>QLNPYLRLKVRRDHIIDDALVRLEMIAMENPADLKKQLYVEFEGEQGVDEGGVSKEFFQLVVEEIFNPDIGMFTYDESTKLFWFNPSSFETEGQFTLIGIVLGLAIYNNCILDVHFPMVVYRKLMGKKGTFRDLGDSHPVLYQSLKDLLEYEGNVEDDMMITFQISQTDLFGNPMMYDLKENGDKIPITNENRKEFVNLYSDYILNKSVEKQFKAFRRGFHMVTNESPLKYLFRPEEIELLICGSRNLD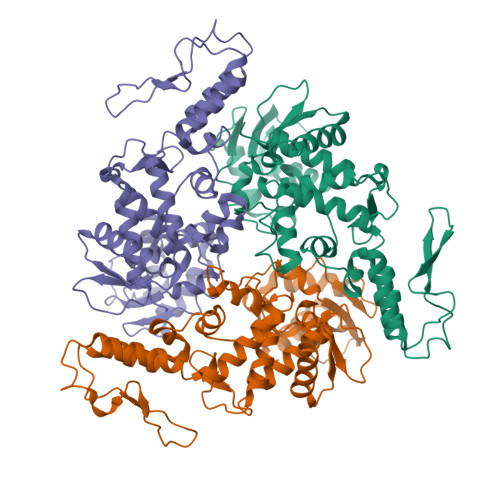FQALEETTEYDGGYTRDSVLIREFWEIVHSFTDEQKRLFLQFTTGTDRAPVGGLGKLKMIIAKNGPDTERLPTSHTCFNVLLLPEYSSKEKLKERLLKAITYAKGFGML[3x]>MTSLAEHTSPNNESSHQRLSEVQKMPTMIEGFDDISHGGLPTGRSTLVSGTSGTGKTLFSIQFLYNGITEFDEPGIFVTFEESPQDIIKNARSFGWNLQKLVDQGKLFILDASPDPDGQEVAGGFDLSALIERINYAIQKYKARRVSIDSVTAVFQQYDAASVVRREIFRLVARLKQIGVTTVMTTERIDEYGPIARYGVEEFVSDNVVILRNVLEGERRRRTVEILKLRGTTHMKGEYPFTINDHGINIFPLGAMRLTQRSSNVRVSSGVPRLDEMCGGGFFKDSIILATGATGTGKTLLVSKFIENACQNKERAILFAYEESRAQLLRNASSWGIDFEEMERQGLLKIICAYPESAGLEDHLQIIKSEIGDFKPSRIAIDSLSALARGVSNNAFRQFVIGVTGYAKQEEITGFFTNTSDQFMGSHSITDSHISTITDTILLLQYVEIRGEMSRAINVFKMRGSWHDKGIREYVITDKGPEIKDSFRNFERIISGSPTRITVDEKSENLSRIARGVQEKEPES[6x]

In this study we reconstruct and analyse the ancient circadian clock system KaiABC (anKaiABC) of cyanobacteria that existed ~0.95 billion years ago, when the daily light/dark cycle was ~18 h-long. KaiC is both an autokinase and an autophosphatase that contains two phosphorylation sites: S431 and T432. KaiC phosphorylation is correlated with the dual adenosine triphosphatase domains located in the CI (1–268 aa) and CII (269–519 aa) regions, respectively. KaiC is the core component in the KaiABC system which can form hexamers; KaiA and KaiB regulate the phosphorylation of KaiC.

Likewise, anKaiC also forms hexamers as revealed by cryo-EM, however, the cryo-EM and SANS results revealed differences in surface hydrophobicity, conformation, and interactions between the ancient and contemporary circadian components. Dispersed differences in the surface hydrophobicity and structure between KaiC and anKaiC were observed. The sequences of the detectable part of the anKaiC A-loop (R492–T499, S-shaped loop) are almost identical to those in KaiC, and they have a very similar structure in this region (Fig. EV1F). However, whether the structure of the remaining C-terminal part (R493–S524) of the A-loop is similar remains unclear because this region is so flexible that the structure cannot be resolved. Differences in the B-loop (A112–D126) and another spatial loop (S150–A160) close to the B-loop were observed, although its function remains elusive. anKaiC harbours two clefts for the binding of ATP molecules in its CI (KaiC-CI) and CII domains, similar to KaiC. Although the inside surface hydrophobicity of anKaiC and KaiC are almost identical (Fig. EV1G), the positions and orientations of the side chain amino acid residues (R165, E187, D206, and R230) surrounding the ATP molecule, showed subtle differences compared with the features of modern KaiC. Moreover, subtle differences in the position and orientation of ATP molecules were also observed. These structural discriminations may lead to functional differences in the catalytic ability of anKaiC as an ATPase, kinase or phosphatase. The ATPase activity of anKaiC is much lower than that of contemporary KaiC, which can be at least in part attributed to the residues T233/N244 spatially neighbouring to ATP molecules.> MEFVAKLFKFFADLLGKF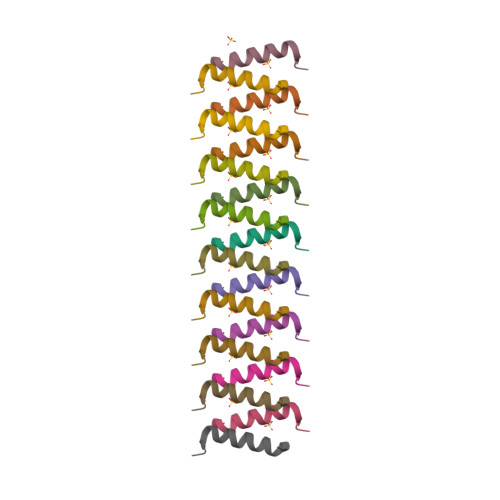LGNN(2,4-DIFLUOROPHENYL)METHANOL 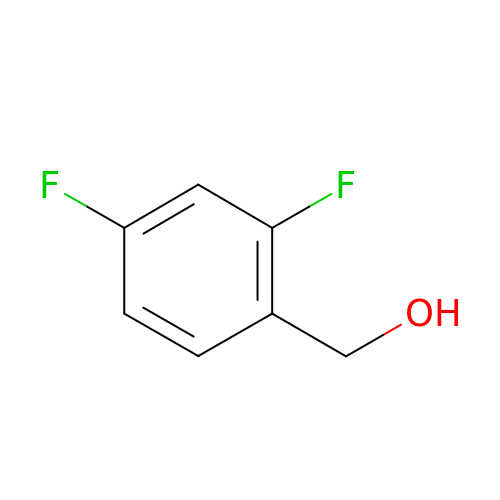| C7 H6 F2 O | NIJZBWHOHNWJBX-UHFFFAOYSA-N>[2x]ADKELKFLVVDDFSTMRRIVRNLLKELGFN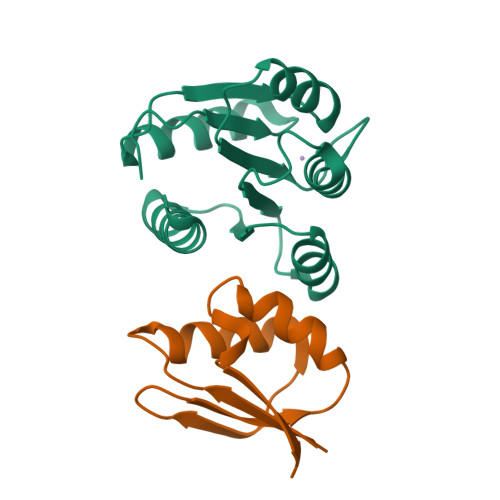NVEEAEDGVDALNKLQAGGYGFVISDWNMPNMDGLELLKTIRADGAMSALPVLMVTAEAKKENIIAAAQAGASGYVVKPFTAATLEEKLNKIFEKLGM;>[2x]RQLALEAKGETPSAVTRLSVVAKSEPQDEQSRSQSPRRIILSRLKAGEVDLLEEELGHLTTLTDVVKGADSLSAILPGDIAEDDITAVLCFVIEADQITFETVEVSPKISTPPVLKLAAEQAPTGRVEREKTTR> MAGLYTTYQLLEVQRKLKTLPAFFLQWFPRQINFQEDMIAFDKVIQDVTRVAPFVAPNVQGRVIKESGYNTKTFKPAYVKPKHVIDPNMIIPRQPGEALGTGTLSIAQRRDRVIAYLLMKHRAMHENTWEWMAAQAAQYGYVDVQGQDYPLVRVDFGRDAALTMTTDWTAAGVTLMDMIADLRDGQRLVSDKSMSGTVIRDYVFGGDAWDQFVKVGGKELWGKDGLMDSTIRGSETNVTRLWDDVEGVQYMGELVGANGAGRMRIW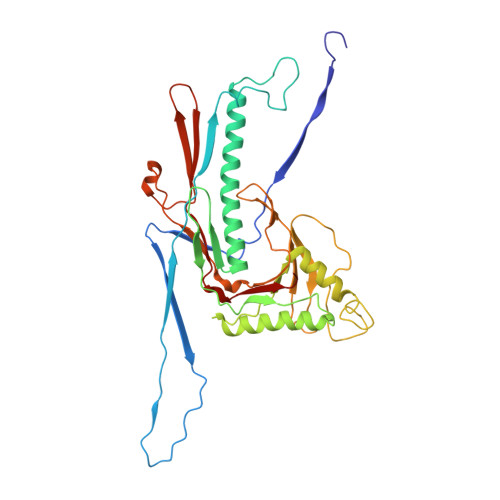VNTQKYRDQNDQEQFLMKQKAVMGISSAIEGVRCFGAILDKGAGYQALDYFPKMWDQEDPSVEYLMSQGAPLMVPADPNASFLLTVMS>LAGLDTAIILIAFIITAAVLAYVAVNMGLFVTQKAKTTINKGEETASTALSLSGNVLYAVNYPTNTKSYWMYFTVSPSSGVSSVDLSPSTTAISFTAASRGVSLSNIYQFSLLSVLPSQVNNKVQVKLGTSIINLTLAFSSNSAGQTYVYYSDPNYALLALNYTLGQEVKGGQLTSSPLYIISNTSIVASKPWLKNDNVFTFNISVNGTEVEYYAYVNKTFAFTYPVSGFPLAGSDIAPAGSVIGVMILFGPGEATNVFQYETVTIQITPNIGSPLTISQYIYQPDGKVTVIG[20x]

While some archaea produce only one type of filament, the archaeal model species Sulfolobus acidocaldarius generates four. These include rotary swimming propellers analogous to bacterial flagella (archaella), pili for twitching motility (Aap), adhesive fibres (threads), and filaments facilitating homologous recombination upon UV stress (UV pili). Here, we use cryo-electron microscopy to describe the structure of the S. acidocaldarius archaellum at 2.0 Å resolution, and update the structures of the thread and the Aap pilus at 2.7 Å and 2.6 Å resolution, respectively. We define distinct N-glycan patterns in the three filaments and identify a putative O-glycosylation site in the thread.

A deletion mutant MW039 (Δagl3), lacking the sulfoquinovose synthase Agl3 generates a trisaccharide N-glycan, missing the sulfoquinovose, one mannose and one glucose molecule. To investigate this, we cultivated the Δagl3 mutant. Moreover, we found that archaella extending from Δagl3 cells still supercoil. Next, we purified archaella and Aap from this mutant and solved their structures by cryoEM. In the maps of the mutant archaellum and Aap, the glycans were clearly altered. The densities for the sulfoqiunovose, the terminal glucose and one mannose were missing. However, comparing the protein structures of the archaella and Aap with and without glycan truncation revealed no significant differences. These findings demonstrate that the motility-reducing effect of the glycan truncation is not due to structural changes in the archaella or Aap. Interestingly however, only the O4-linked α-mannose was missing from the N-glycan trees of the Δagl3 filaments, while the O6-linked α-mannose was still present. However, S. acidocaldarius Δagl3 mutants were virtually non-motile, indicating that glycosylation is important for archaellum driven motility in S. acidocaldarius.FILIA is a member of a recently identified oocyte/embryo expressed family whose members are characterized by an atypical KH domain. The SCMC contains a core formed by FLOPED, MATER, TLE6, and FILIA. FILIA is important in regulation of mitotic kinase activity and spindle assembly checkpoint activation, and contributes to chromosome stability, although the molecular basis for the relationship between its special localization and its unique function is not clear. In order to study the structural basis for its function, we expressed and crystallized the N-terminal domain of FILIA ranging from 1 to 124 amino acids (named FILIA-N hereafter).

The crystal structure of FILIA-N (1–124 AA) was solved by the single wavelength anomalous diffraction (SAD) method. FILIA-N crystallized with two molecules in an asymmetric unit forming a stable dimer. From residues 40–118, FILIA-N forms a classical KH module with a β-α-α-β-β-α topology. The N-terminal 39 residues prior to the KH region form a unique substructure in FILIA-N. This substructure is composed of a loop at the beginning (residues 2-12), followed by two anti-parallel β-strands (β-1 and β0) and an α-helix (α0). The peptide from residues 2–12 is located in a groove formed by the β-1-β0-sheet and the β1-β2-β3 sheet, bridging the N-terminal extension and canonical KH region, thus contributing towards the stability of the whole molecule. The total buried area in the dimer of FILIA-N was approximately 1920 Å2 compared to 930 Å2 for the Nova2-KH3 dimer. On the dimerization surface, most of the interactions involve the helices α2 and α3. Hydrophobic interactions contribute most of the stabilizing forces, including residues Met68, Met101, Leu65, Leu69, and Leu105. A measured molecular mass of 29814 Da was obtained with a Kd of 10 nM, indicating a stable dimer with high affinity. Surprisingly, although the FILIA 40–124 (FILIA-NΔ39) protein lacking the N-terminal extension still possessed a KH domain, it completely lost the ability to bind RNA.

>[2x]MHHHHHHENLYFQSNAMASLKRFQTLVPLDHKQGTLFEIIGEPKLPKWFHVECLEDPKRLYVEPRLLEIMFGKDGEHIPHLESMLHTLIHVNVWGPERRAEIWIFGPPPFRRDVDRMLTDLAHYCRMKLMEIEALEAGVE>[2x]MKEEKRSSTGFLVKQRAFLKLYMI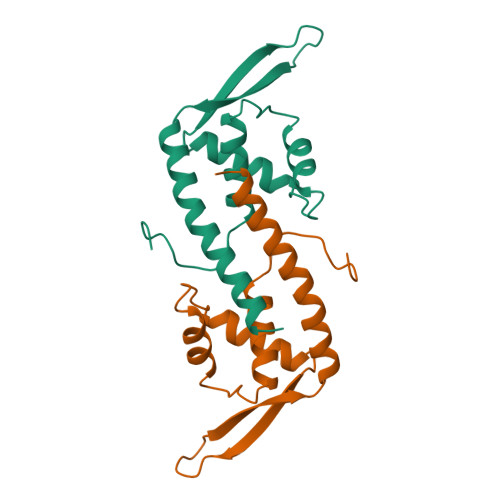TMTEQERLYGLKLLEVLRSEFKEIGFKPNHTEVYRSLHELLDDGILKQIKVKKEGAKLQEVVLYQFKDYEAAKLYKKQLKVELDRCKKLIEKALSDNF> KDSAPRKPAEEPSPSVGEARPEPAKAEEKPAEPVSRPTKVVKTPVRGGMQIYAAGGDLIVLAAVSPGAELLADGNIHVYGPMRGRALAGVKGDATARIFCQQLAAELVSIAGNYKVA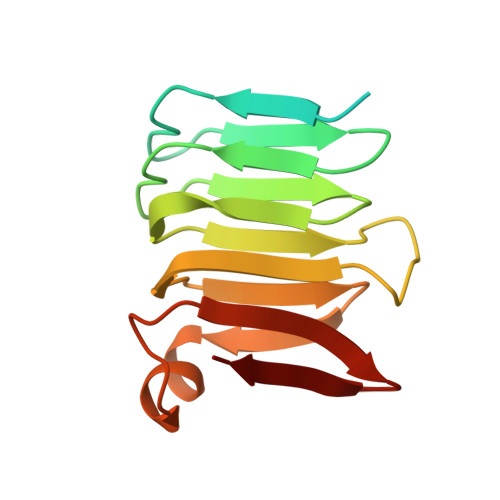EDLRRSPQWGKAVHVSLSGDVLNITRL> SLGAKPFGEKKFIEIKGRRMAYIDEGTGDPILFQHGNPTSSYLWRNIMPHCAGLGRLIACDLIGMGDSDKLDPSGPERYAYAEHRDYLDALWEALDLGDRVVLVVHDWGSALGFDWARRHRERVQGIAYMEAIAMPIEAADLPEQDRDLFQAFRSQAGEELVLQDNVFVEQVLPGWILRPLSEAEMAAYREPFLAAGEARRPTLSWPRQLPIAG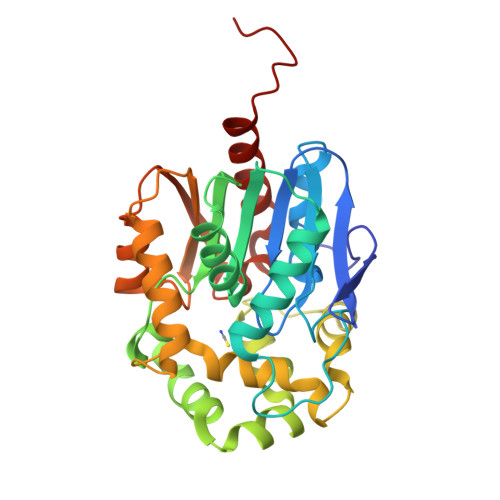TPADVVAIARDYAGWLSESPIPKLFINAEPGALTTGRMRDFCRTWPNQTEITVAGAHFIQEDSPDEIGAAIAAFVRRLRPAHHHHHH In this study, we focus on the ω-transaminase from Mycobacterium vanbaalenii (MvTA) which exhibits activity toward d-fructose rather than fructose 6-phosphate. The transaminase MvTA demonstrates transaminate activity toward d-fructose 1, and the resulting 2-amino-2-deoxy-mannitol (ADM) 2 undergoes dehydrogenation under the enzyme GutB1 and spontaneously cyclizes to produce the valuable azasugar mannojirimycin (MJ), which serves as a precursor for 1-DNJ. The dimeric enzyme exhibited the characteristic structural architecture of class IV PLP-dependent enzymes, consisting of two subunits. The interface between the two subunits constituted the binding pocket for the amino donor and acceptor.

A mutant M9 with significantly enhanced activity and thermostability has been successfully obtained and crystallized for structural resolution. The obtained mutant M9, incorporating nine mutation sites, exhibited a remarkable 16.4-fold increase in specific activity and an impressive 208-fold improvement in thermostability compared to WT. In all three structures, the asymmetric unit comprised two polypeptide chains forming a homodimer. Moreover, the mutation of K142P notably heightened the rigidity of the loop region (137–146). In both the first and second half-reactions, the RMSF values for the loop region (102–108) and its adjacent α-helices in M9 were notably lower compared to WT. These findings indicated that the proline substitution at position 105 could enhance the rigidity of the loop region, consequently reducing the flexibility of its neighboring α-helices.

>[2x]MGIDTGTSNLVAVEPGAIREDTPAGSVIQYSDYEIDYSSPFAGGVAWIEGEYLPAEDAKISIFDTGFGHSDLTYTVAHVWHGNIFRLGDHLDRLLDGARKLRLDSGYTKDELADITKKCVSLSQLRESFVNLTITRGYGKRKGEKDLSKLTHQVYIYAIPYLWAFPPAEQIFGTTAVVPRHVRRAGRNTVDPTIKNYQWGDLTAASFEAKDRGARTAILMDADNCVAEGPGFNVCIVKDGKLASPSRNALPGITRKTVFEIAGAMGIEAALRDVTSHELYDADEIMAVTTAGGVTPINTLDGVPIGDGEPGPVTVAIRDRFWALMDEPGPLIEAIQY RETINOL 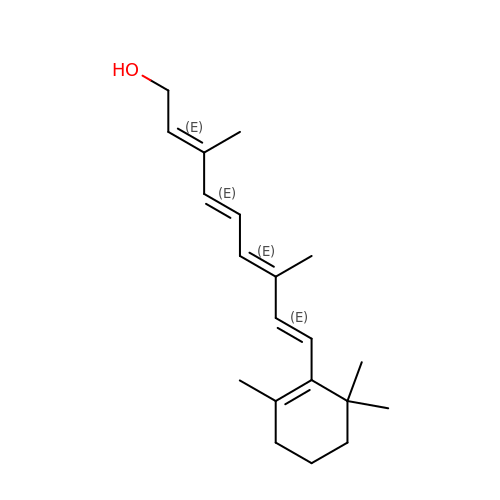| C20 H30 O | FPIPGXGPPPQFEQ-OVSJKPMPSA-N> RDFNNLTKGLCTINSWHIYGKDNAVRIGEDSDVLVTREPYVSCDPDECRFYALSQGTTIRGKHSNGTIHDRSQYRALISWPLSSPPTVYNSRVECIGWSSTSCHDGKTRMSICISGPNNNASAVIWYNRRPVTEINTWARNILRTQESECVCHNGVCPVVFTDGSATGPAETRIYYFKEGKILKWEPLAGTAKHIEECSCYGERAEITCTCRDNWQGSNR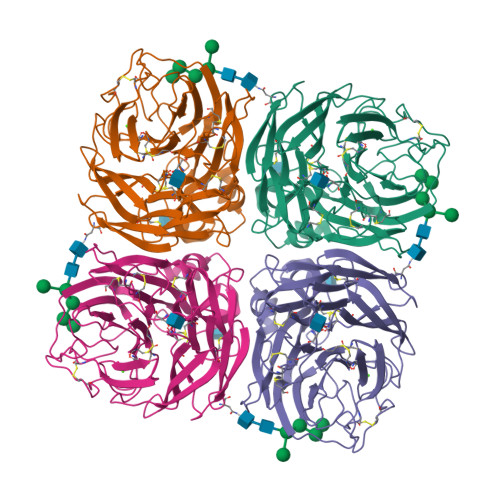PVIRIDPVAMTHTSQYICSPVLTDNPRPNDPTVGKCNDPYPGNNNNGVKGFSYLDGVNTWLGRTISRASRSGYEMLKVPNALTDDKSKPTQGQTIVLNTDWSGYSGSFMDYWAEGECYRACFYVELIRGRPKEDKVWWTSNSIVSMCSSTEFLGQWDWPDGAKIEYFL>[2x]SMGVHSFWDIAGPTARPVRLESLEDKRMAVDASIWIYQFLKAVRDQEGNAVKNSHITGFFRRICKLLYFGIRPVFVFDGGVPVLKRETIRQRKERRQGKRESAKSTARKLLANTTLSTSAERNVAENAFVEDELFEQQMKDKRDSDEVTMDMIKEVQELLSRFG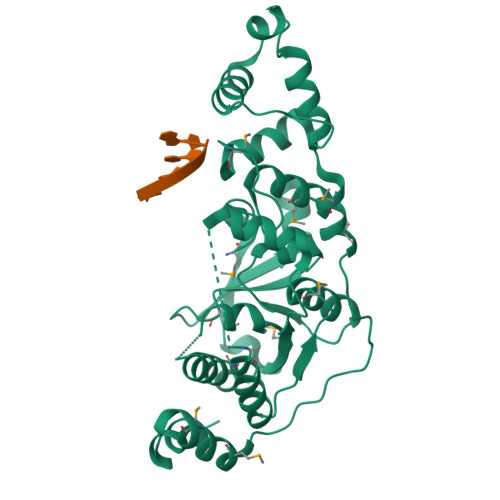IPYITAPMEAEAQCAELLQLNLVDGIITDDSDVFLFGGTKIYKNMFHEKNYVEFYDAESILKLLGLDRKNMIELAQLLGSDYTNGLKGMGPVSSIEVIAEFGNLKNFKDWYNNGQFDKRKQETENKFEKDLRKKLVNNEIILDDDFPSVMVYDAYMRPEVDHDTTPFVWGVPDLDMLRSFMKTQLGWPHEKSDEILIPLIRDV>[4x]FACKTANGTAIPIGGGSANVYVNLAPVVNVGQNLVVDLSTQIFCHNDYPETITDYVTLQRGSAYGGVLSNFSGTV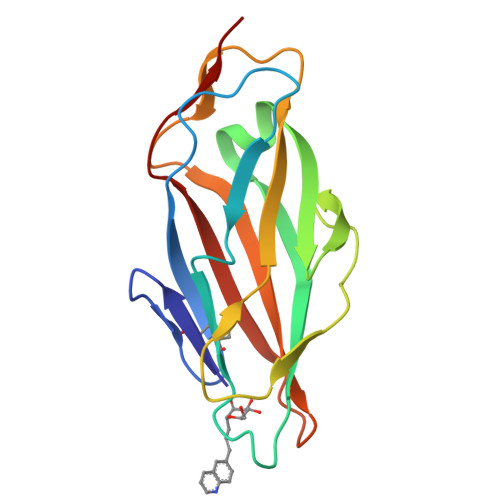KYSGSSYPFPTTSETPRVVYNSRTDKPWPVALYLTPVSSAGGVAIKAGSLIAVLILRQTNNYNSDDFQFVWNIYANNDVVVPT>[2x]MSKIRVLSVDDSALMRQIMTEIINSHSDMEMVATAPDPLVARDLIKKFNPDVLTLDVEMPRMDGLDFLEKLMRLRPMPVVMVSSLTGKGSEVTLRALELGAIDFVTKPQLGIREGMLAYSEMIAEKVRTAARARIAAHKPMAAPTTLKAGPLLSSEKLIAIGASTGGTEAIRHVLQPLPLSSPAVIITQHMP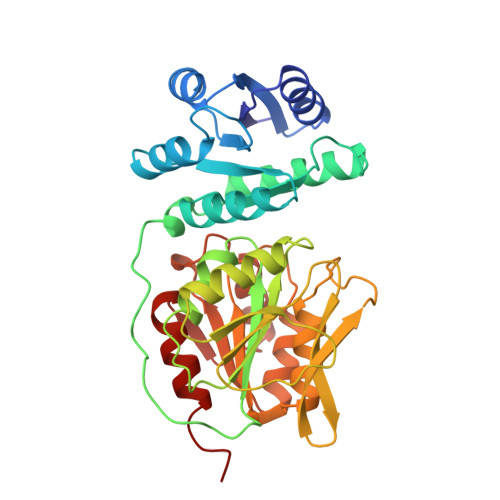PGFTRSFAERLNKLCQISVKEAEDGERVLPGHAYIAPGDKHMELARSGANYQIKIHDGPPVNRHRPSVDVLFHSVAKHAGRNAVGVILTGMGNDGAAGMLAMYQAGAWTIAQNEASCVVFGMPREAINMGGVSEVVDLSQVSQQMLAKISAGQAIRI The final step in the pathway is catalyzed by a 2-epimerase, which utilizes UDP-2,3-diacetamido-2,3-dideoxy-d-glucuronic acid as its substrate. The focus of this investigation is on the ORF WP_011172736, which we demonstrate encodes for a 2-epimerase. We have also demonstrated that the T. thermophilus enzyme is allosterically regulated by UDP-GlcNAc. Whereas the sugar 2-epimerases that function on UDP-GlcNAc have been the focus of past biochemical and structural analyses, this is the first detailed investigation of a 2-epimerase that specifically utilizes UDP-2,3-diacetamido-2,3-dideoxy-d-glucuronic acid as its substrate.

The first structure determined in this investigation was that of the apoenzyme crystallized at pH 9.0 (structure 1). The crystals of the protein belonged to the P21 space group with two subunits in the asymmetric unit. The model was refined at 2.3 Å resolution with an overall R-factor of 20.1%. The two subunits superimpose with an RMSD of 0.6 Å. Each subunit adopts a bilobal architecture with domain 1 defined by Met 1 to Val 170 and domain 2 formed by Gly 171 to Gly 346. The architecture of domain 1 is dominated by a seven-stranded parallel β-sheet flanked on either side by a total of six α-helices. Domain 2 contains a six-stranded parallel β-sheet surrounded by nine α-helices. The final α-helix, formed by Ala 350 to Lys 360, extends from domain 2 back to domain 1. The total buried surface area for the dimer is ∼2850 Å2. The subunit:subunit interface is primarily formed by three α-helices defined by His 70 to Glu 88, Thr 99 to Lys 111, and Pro 131 to Ala 142 in subunit A running antiparallel to the same α-helices in subunit B. As shown in Figure 4B, the interface is fairly hydrophobic in nature with Leu 78, Leu 103, Leu 107, Val 110, and Leu 138 projecting inward.

>[2x]GHMWVKILSVVGARPQFIKAAAVSRVLRASPGVREVLVHTGQHYDDNMSQVFFEELEIPDPDYHLGIGGGTHGQNTGRMLEAIEGVLLKEKPDWVLVYGDTDSTLAGALAAVKLHIPVAHVEAGLRSFNRRMPEEINRILTDHASDLLFAPTETAVQNLLREGIPENRIHLVGDVMYDAALHYGAKAERKSRILERLGLQAKGYVLATIHRAENTDDQERLRVILEALAEVHQEVPVVFPVHPRTRKRAEAFGLGSYLEKVVALEPVGYLDMVMLEKNARLIVTDSGGVQKEAYFYRVPCVTVREETEWVELLKAEWNYLAAPQNAKDLALTILHRMRTKGVEIDLYGDGRASQKISDFLRKVGIRT> MPIMLEDYQKNFLELAIECQALRFGSFKLKSGRESPYFFNLGLFNTGKLLSNLATAYAIAIIQSDLKFDVIFGPAYKGIPLAAIVCVKLAEIGGSKFQNIQYAFNRKEAKDHGEGGIIVGSALENKRILIIDDVMTAGTAINEAFEIISNAKGQVVGSIIALDRQEVVSTDDKEGLSATQTVSKKYGIPVLSIVSLIHIITYLEGRITAEEKSKIE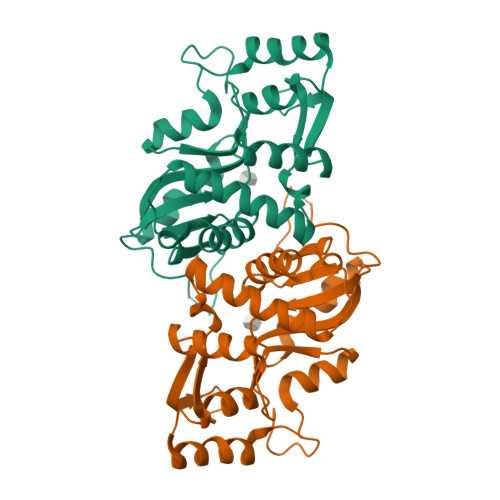QYLQTYGASAENLYFQ>MAPVQGSYDYDLIVIGGGSAGLACAKEAVLNGARVACLDFVKPTPTLGTKWGVGGTCVNVGCIPKKLMHQASLLGEAVHEAAAYGWNVDDKIKPDWHKLVQSVQNHIKSVNWVTRVDLRDKKVEYINGLGSFVDSHTLLAKLKSGERTITAQTFVIAVGGRPRYPDIPGAVEYGITSDDLFSLDREPGKTLVVGAGYIGLECAGFLKGLGYEPTVMVRSIVLRGFDQQMAELVAASMEERGIPFLRKTVPLSVEKQDDGKLLVKYKNVETGEESEDVYDTVLWAIGRKGLVDDLNLPNAGVTVQKDKIPVDSQEATNVANIYAVGDIIYGKPELTPVAVLAGRL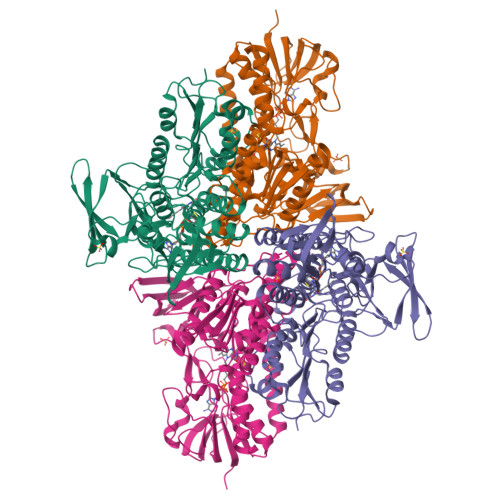LARRLYGGSTQRMDYKDVATTVFTPLEYACVGLSEEDAVKQFGADEIEVFHGYYKPTEFFIPQKSVRYCYLKAVAERHGDQRVYGLHYIGPVAGEVIQGFAAALKSGLTINTLINTVGIHPTTAEEFTRLAITKRSGLD[2x]>MAHHHHHHRSSTT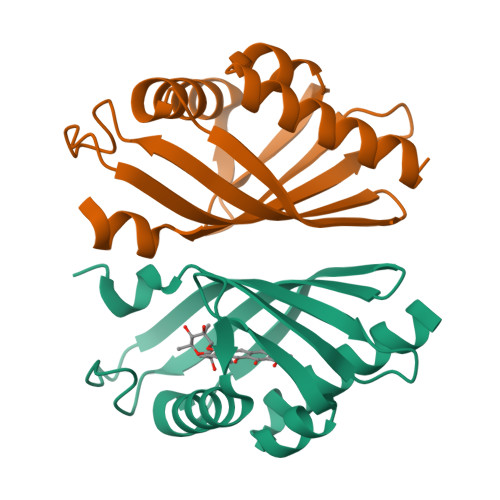ANKERCLEMVAAWNRWDVSGVVAHWAPDVVHYDDEDKPVSAEEVVRRMNSAVEAFPDLRLDVRSIVGEGDRVMLRITCSATHQGVFMGIAPTGRKVRWTYLEELRFSEAGKVVEHWDVFNFSPLFRDLGVVPDGL[2x]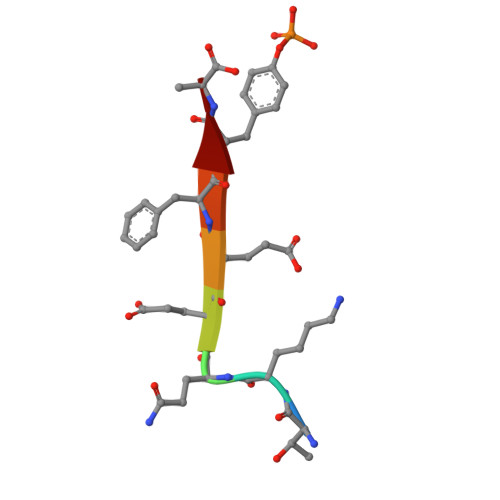> TKQEEFYA>SNAMKDFHFDAISAFENYEIEKMRDGHVVVTTKVVNSSLNYYGNAHGGYLFTLCAQISGLVVISLGLDG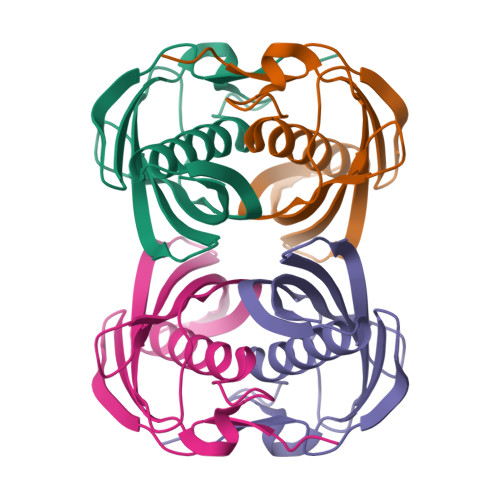VTLQSSINYLKAGKLDDVLTIKGECVHQGRTTCVMDVDITNQEGRNVCKATFTMFVTGQRSEERRVRI[2x]> DDGTGQKQIWRIEGSNKVPVDPATYGQFYGGDSYIILYNYRHGGRQGQIIYNWQGAQSTQDEVAASAILTAQLDEELGGTPVQSRVVQGKEPAHLMSLFGGKPMIIYKGGTSRDGGQTAPASIRLFQVRASSSGATRAVEVMPKSGALNSNDAFVLKTPSAAYLWVGAGASEAEKTAAQELLKVLRSQHVQVEEGSEPDGFWEALGGKTSYRTSPRLKDKKMDAHPPRLFACSNRIGRFVIEEVPGELMQEDLATDDVMLLDTWDQVFVWVGKDSQEEE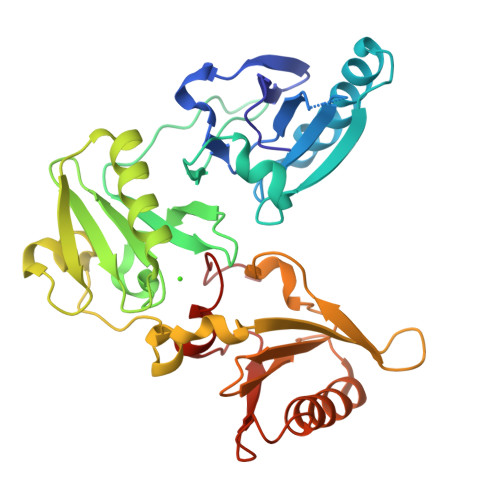KTEALTSAKRYIETDPANRDRRTPITVVRQGFEPPSFVGWFLGWDNNYWS>[2x]MAHHHHHHVGTFENITAAPADPILGLADLFRADERPGKINLGIGLYYDETGKIPVLT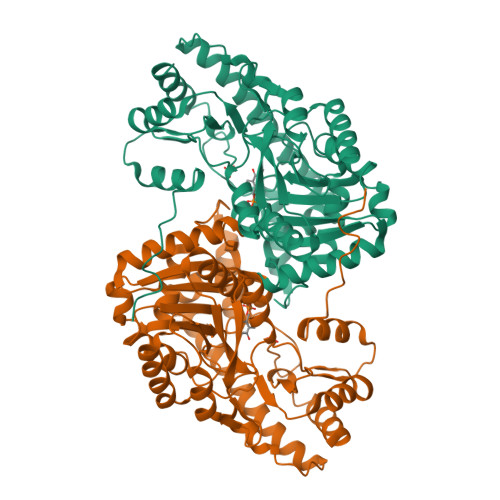SVKKAEQYLLENETTKLYLGIDGIPEFGRCTQELLFGKGSALINDKRARTAQTPGGSGALRVAADFLAKNTSVKRVWVSNPSWPNHKSVFNSAGLEVREYAYYDAENHTLDFDALINSLNEAQAGDVVLFHGCCHNPTGIDPTLEQWQTLAQLSVEKGWLPLFDFAYQGFARGLEEDAEGLRAFAAMHKELIVASSYSKNFGLYNERVGACTLVAADSETVDRAFSQMKAAIRANYSSPPAHGASVVATILSNDALRAIWEQELTDMRQRIQRMRQLFVNTLQEKGANRDFSFIIKQNGMFSFSGLTKEQVLRLREEFGVYAVASGRVNVAGMTPDNMAPLCEAIVAVL ArdK is a 102 amino acid protein encoded by the broad host range conjugative plasmid R388. In R388, ArdK represses the expression of five genes by its binding to their respective promoters (PardC, Porf7, Pssb, Porf12 and Porf14). The KorA family of transcriptional regulators includes plasmid-borne repressors involved in plasmid stability and conjugation. Our structural analyses show that ArdK, a member of this family, can form a symmetric dimer similar to that observed for KorA, yet it binds direct sequence repeats as a non-symmetric dimer.

To study the structural changes involved in this alternative binding mode, we obtained the crystal structure of ArdK bound to an IR with an n = 3 loop, as described in the Materials and Methods. Strikingly, the IR–ArdK complex did not show any significant structural change compared with the DR–ArdK structure previously obtained. Despite the palindromic structure of the operator, the protein binds in a head-to-tail configuration. Furthermore, a close inspection of the DNA–protein contacts indicated that the DNA–protein interface was formed by the same amino acids. The –35 box was again recognized by the rotating HTH motif, while the fixed HTH recognized the same GC base pair. The structure revealed the reason why ArdK was able to recognize that particular IR configuration: the n = 3 loop maintained the adventitious TGxCA repeat at the same distance as in its cognate DR architecture. Bases located in between were different, but these were only contacted through their sugar backbone. Thus, although the operator had an apparent palindromic structure, it was contacted and recognized as a degenerate DR. The distance between the IR arms was necessary to situate the bases specifically recognized by each HTH domain (a GC pair) at the same distance as in the DR configuration. The results thus demonstrate that a TF may recognize operators with a DR or IR apparent topology without changes in the DNA binding mechanism.

>[2x]MTAAAFDDLRPRLGRLTEETIDIAREVLVEGKSQSDVARERGLSRQRVSSMVKSVVSAANEIPREWQRVEVWLPPNLAEKVRQMEADAKADVARKNQLTDAALEHHHHHH>XEVEALEAKVEALESKVQKLEKKVEALEHGWD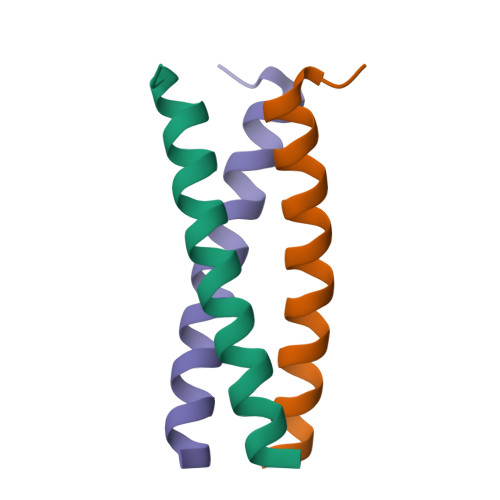[2x]> DRHHHHHHKLSPPAAPRFNVSLDSVPELRWLPVLRHYDLDLVRAAMAQ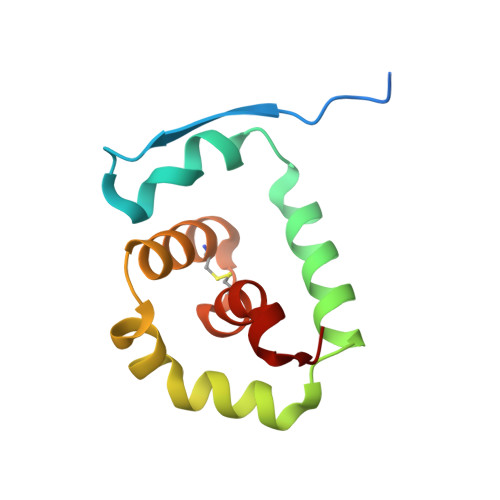VIGDRVPKWVHVLIGKVVLELERFLPQPFTGEIRGMCDFMNLSLADCLLVNLAYESSVF> PTLSPEQQEMLQAFSTQSGMNLEWSQKCLQDNNWDYT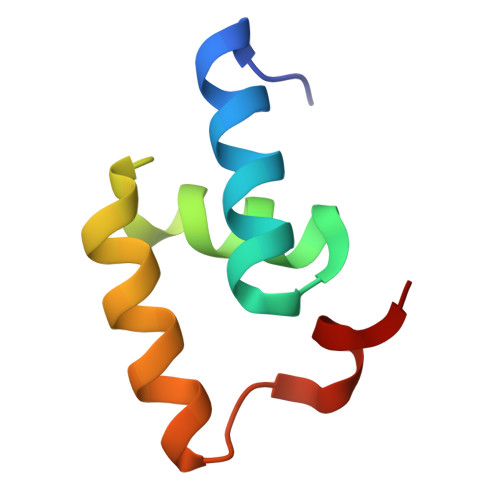RSAQAFTHLKAKGEIPEVAFMK>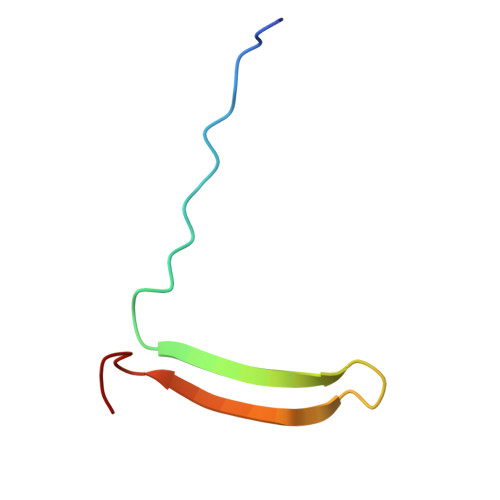 LEAIPRSIPPEVKFNAPFVFLMIEQNTKSPLFMGKVVNPTQK>GSKFSAKRLPSTRLGTFLENRVNDFLRRQNHPESGEVTVRVVHASDKTVEVKPGMKARFVDSGEMAESFPYRTKALFAFEEIDGVDLCFFGMHVQEYGSDCPPPNQRRVYISYLDSVHFFRPKCLRTAVYHEILIGYLEYVKKLGYTTGHIWACPPSEGDDYIFHCHPPDQKIPKPKRLQEWFKKMLDKAVSERIVHDYKDIFKQATEDRLTSAKELPYFEGDFWPNVLEESIKESGGSGSQKLYATMEKHKEVFFVIRLIAGPAANSLPPIVDPDPLIPCDLMDGRDAFLTLARDKHLEFSSLRRAQWSTMCMLVELHTQSQ[2x]

P300 is an ∼2400AA multidomain protein whose catalytic core consists of bromo-, RING, PHD, and histone acetyltransferase (HAT) domains. By acetylating histones, p300 promotes gene expression. It can also acetylate itself, as well as other proteins, and recruit a larger complex of proteins including transcription factors. The overall structure is as expected from previous p300-HAT structures: a central β-sheet is composed of seven β-strands and surrounded by nine α-helices.

To improve homogeneity, a construct omitting the autoacetylation-prone autoinhibitory loop was inactivated through mutation of residue Y1467 to F: p300‐HAT‐YF‐Δloop [K1287‐Q1663/Y1467F/Δ(L1520‐L1580)] and overexpressed in E. coli. Blade-form ternary crystals of p300‐HAT‐YF‐Δloop with CoA and CPI-076 were obtained at 4° C from 200 + 150 nl microseeded sitting drops with a 60 μl reservoir consisting of 20% MPD, 0.1M Tris pH 8, and 7.5% PEG 5000 MME. Despite their chemical differences, these new allosteric compounds bind in the same location, ∼8 Å distant from the active site, between the α5 and α6 helices. So though these compounds are AcCoA modulated, there is obviously no direct competition for the AcCoA binding site. CPI-076 is secured in p300-HAT-CoA by hydrophobic interactions and a hydrogen bond with Asp1507 and also creates a water network out to Arg1392/Ile1486. With CPI-076's measured HAT-domain IC50 20 μM, SBDD efforts focused on driving the biochemical activity. CPI-076's structure offered 2 potential vectors for compound elaboration [Fig. 6(a)]. However, derivatization failed to improve the compound activity from this starting point (data not shown). The related compound CPI-076 had no measurable FL activity.> MPLNRTLSMSSLPGLEDWEDEFDLENAVLFEVAWEVANKVGGIYTVLQTKAKVTGDEWGDNYFLVGPYTEQGVRTQVELLEAPTPALKRTLDSMNSKGCKVYFGRWLIEGGPLVVLLDVGASAWALERWKGELWDTC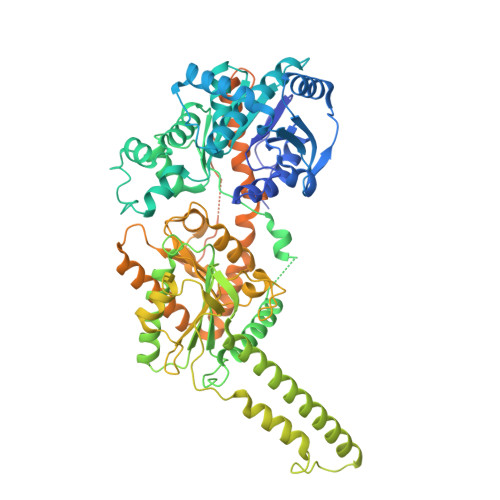NIGVPWYDREANDAVLFGFLTTWFLGEFLAQSEEKPHVVAHFHEWLAGVGLCLCRARRLPVATIFTTHATLLGRYLCAGAVDFYNNLENFNVDKEAGERQIYHRYCMERAAAHCAHVFTTVSQITAIEAQHLLKRKPDIVTPNGLNVKKFSAMHEFQNLHAQSKARIQEFVRGHFYGHLDFNLDKTLYFFIAGRYEFSNKGADVFLEALARLNYLLRVNGSEQTVVAFFIMPARTNNFNVETLKGQAVRKQLWDTANTVKEKFGRKLYESLLVGSLPDMNKMLDKEDFTMMKRAIFATQRQSFPPVCTHNMLDDSSDPILTTIRRIGLFNSSADRVKVIFHPEFLSSTSPLLPVDYEEFVRGCHLGVFPSYYEPWGYTPAECTVMGIPSISTNLSGFGCFMEEHIADPSAYGIYILDRRFRSLDDSCSQLTSFLYSFCQQSRRQRIIQRNRTERLSDLLDWKYLGRYYMSARHMALSKAFPEHFTYEPNEADAAQGYRYPRPASVPPSPSLSRHSSPHQSEDEEDPRNGPLEEDGERYDEDEEAAKDRRNIRAPEWPRRASCTSSTSGSKRNSVDTATSSSLSTPSEPLSPTSSLGEERN PIPERAZINE-N,N'-BIS(2-ETHANESULFONIC 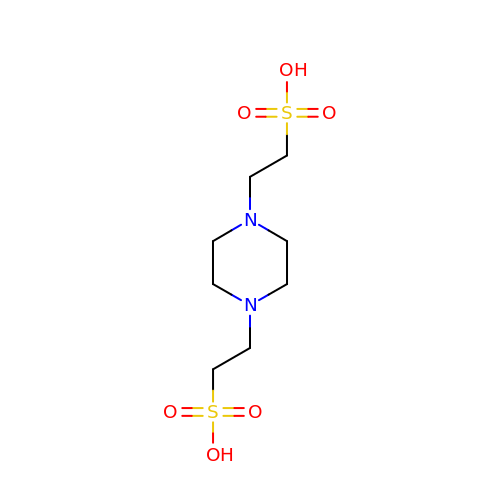ACID) | C8 H18 N2 O6 S2 | IHPYMWDTONKSCO-UHFFFAOYSA-N> MVDFIPVENLETTMRSPVFTDNSSPPAVPQSFQVAHLHAPTGSGKSTKVPAAYAAQGYKVLVLNPSVAATLGFGAYMSKA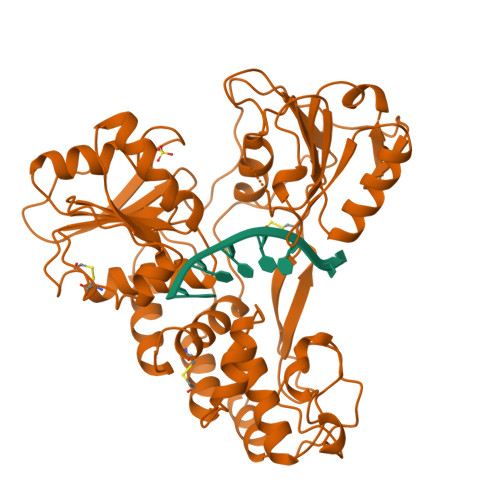HGVDPNIRTGVRTITTGSPITYSTYGKFLADGGCSGGAYDIIICDECHSTDATSILGIGTVLDQAETAGARLVVLATATPPGSVTVPHPNIEEVALSTTGEIPFYGKAIPLEVIKGGRHLIFCHSKKKCDELAAKLVALGINAVAYYRGLDVSVIPTSGDVVVVATDALMTGFTGDFDSVIDCNTCVTQTVDFSLDPTFTIETTTLPQDAVSRTQRRGRTGRGKPGIYRFVAPGERPSGMFDSSVLCECYDAGCAWYELTPAETTVRLRAYMNTPGLPVCQDHLEFWEGVFTGLTHIDAHFLSQTKQSGENFPYLVAYQATVCARAQAPPPSWDQMWKCLIRLKPTLHGPTPLLYRLGAVQNEVTLTHPITKYIMTCMSADLEVVTGSGSHHHHHH> MNCRS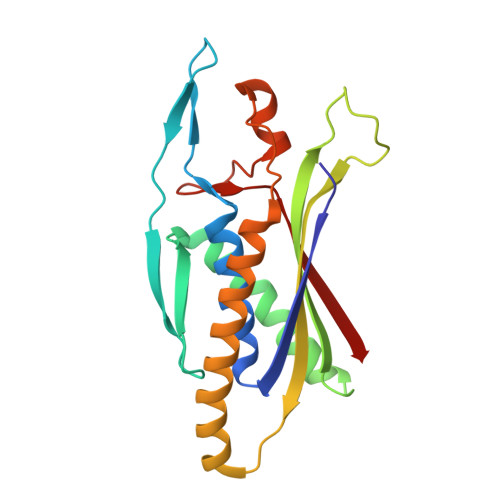EVLEVSVEGRQVEEAMLAVLHTVLLHRSTGKFHYKKEGTYSIGTVGTQDVDCDFIDFTYVRVSSEELDRALRKVVGEFKDALRNSGGDGLGQMSLEFYQKKKSRWPFSDECIPWEVWTVKVHVVALATEQERQICREKVGEKLCEKIINIVEVMNRHEYLPKMPTQSEVDNVFDTGLRDVQPYLYKISFQITD>[3x]APARPAHPLDPLSTAEIKAATNTVKSYFAGKKISFNTVTLREPARKAYIQWKEQGGPLPPRLAYYVILEAGKPGVKEGLVDLASLSVIETRALETVQPILTVEDLCSTEEVIRNDPAVIEQCVLSGIPANEMHKVYCDPWTIGYDERWGTGKRLQQALVYYRSDEDDSQYSHPLDFCPIVDTEEKKVIFIDIPNRRRKVSKHKHANFYPKHMIEKVGAMRPEAPPINVTQPEGVSFKMTGNVMEWSNFKFHIGFNYREGIVLSDVSYNDHGNVRPIFHRISLSEMIVPYGSPEFPHQRKHALDIGEYGAGYMTNPLSLGCDCKGVIHYLDAHFSDRAGDPITVKNAVCIHEEDDGLLFKHSDFRDNFATSLVTRATKLVVSQIFTAANYEYCLYWVFMQDGAIRLDIRLTGILNTYILGDDEEAGPWGTRVYPNVNAHNHQHLFSLRIDPRIDGDGNSAAACDAKSSPYPLGSPENMYGN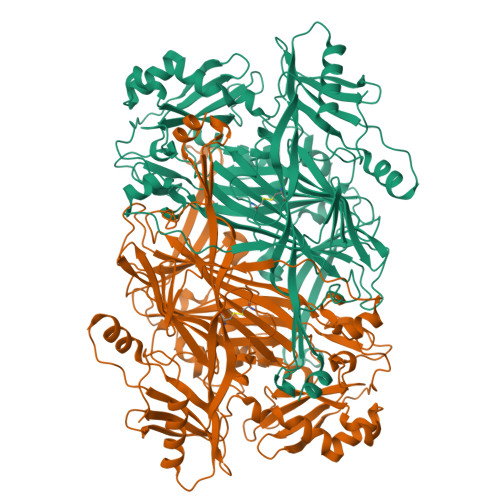AFYSEKTTFKTVKDSLTNYESATGRSWDIFNPNKVNPYSGKPPSYKLVSTQCPPLLAKEGSLVAKRAPWASHSVNVVPYKDNRLYPSGDHVPQWSGDGVRGMREWIGDGSENIDNTDILFFHTFGITHFPAPEDFPLMPAEPITLMLRPRHFFTENPGLDIQPSYAMTTSEAKRAV>MAGAAAAVTVEEVRKAQRASGPATVLAIGTATPANCVHQADYPDYYFRVTKSDHLTDLKEKFKRMCDKSMIRKRYMHLTEEFLAENPNMCAYMAPSLDARQDIVVVEVPKLGKAAAQKALKEWGQPRSRITHLVFCTTSGVDMPGADYQLTKLLGLRPSVNRLMMYQQGCFAGGTVLRVAKDLAENNRGARVLVVCSEITAVTFRGPSESHLDSLVGQALFGDGAAAVIVGADPDERAERPLFQLVSAAQTLLPDSEGAIDGHLREVGLTFHLLKDVPGLISKNIERALEAAFAPLGISDWNSIFWVAHPGGPAILDQVEAKVSLDKARMRATRHVLAEYGNMSSACVLFILDEMRKRSAEDGCATTGEGLDWGVLFGFGPGLTVETVVLHSVPITAGAAAA[4x]

Chalcone synthase (CHS) and chalcone isomerase (CHI) catalyze the first two committed steps of the flavonoid pathway that plays a pivotal role in the growth and reproduction of land plants, including UV protection, pigmentation, symbiotic nitrogen fixation, and pathogen resistance. Based on the obtained X-ray crystal structures of CHS, CHI, and chalcone isomerase-like protein (CHIL) from the same monocotyledon, Panicum virgatum, along with the results of the steady-state kinetics, spectroscopic/thermodynamic analyses, intermolecular interactions, and their effect on each catalytic step are proposed. The production of these value-added products also offers the prospect of increasing the value of the crop, especially because many of these compounds are soluble and readily extracted. This study characterized the enzymes involved in the first two committed steps of the flavonoid pathway, CHS and CHI, and the non-catalytic protein CHIL. Through crystal structure, molecular docking, mutagenesis, kinetic analyses, ITC, and FRET analysis, our study provides evidence supporting a revised catalytic reaction mechanism for monocot CHS and CHI and identified an intermolecular interaction of CHS with both CHI and CHIL in a non-competitive manner.

The crystal lattice packing indicated that four molecules in the triclinic unit cell were composed of two closely associated homodimers. The two PvCHS subunits in each dimer established a dimer interface with 32 hydrogen bonds and 17 salt bridges, suggesting that PvCHS likely exists as a homodimer in a cellular environment. The electron density corresponding to an extended CoA molecule along a continuous tunnel piercing deeply into the PvCHS molecule was visible from an early refinement stage in only the A and C subunits. At the equivalent regions of the dimeric partners, the B and D subunits, the same tunnels were visible with only crystallographic waters near the active site. The overall structure of apo-form PvCHS was not altered significantly upon binding CoA molecules. The only noticeable difference between apo-form (B and D subunits) and CoA binary complex (A and C subunits) PvCHS was the conformation of a short loop, 271FHLLKD276 near the adenosyl and thiol groups of the bound CoA molecule, which appeared to stabilize the bent CoA confirmation described below. Especially, as observed in CHSs of euphyllophytes, the sidechain of Cys-170 displayed extra electron density and was fit with cysteine sulfinic acid, which indicates its enhanced nucleophilicity and susceptibility to oxidation. In addition to a bound CoA molecule, one naringenin molecule was visible in the concave pocket established at the interface between two PvCHS dimers in a stacked orientation of the A and C rings from each naringenin molecule.>[4x]MASMHVYILFAHPSRKSFSREVLEAFTEGLSEAGHTYEVGDLYRMNFRSELSQEEY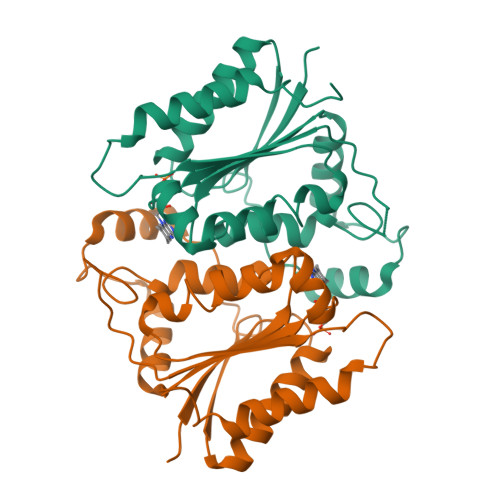LREISQEAGSPLPEDVMEEHERIGRADALAFIYPLWWSDCPAKLKGWFDRVWTYGYAYFYEDGERGTRIDIEKAVVLCSAGHTEEDLEGTGIAESMRSVMLGDRLLGVGVKNVTMEILGGMVPGDDSCREINLMRARRAGRNLEHHHHHH>[3x]GHMWPSAKFIDGRVAFSRMPAERELDEVARDFDAVVVLVEDYELPYSLDEWEKRGVEVLHGPIPDFTAPSVEQLLEILRWIEERVREGKKVLIHCMGGLGRSGTVGVAWLMYSRGLSLREALMEVRRKRPGAVETQEQMEVLKELEERI

In this study, we report the crystal structures of three forms of Tk-PTP, which showed that this protein forms a canonical DUSP fold and that it undergoes an atypical temperature-dependent conformational change between two forms. Structural and biochemical analyses revealed that this structural alteration requires the presence of the GG motif in the P-loop, and that Tk-PTP has dual amino acids, Asp63 and Glu132, both functioning as the general acid/base residues. PTP proteins commonly share a highly conserved active site motif called the PTP signature motif, which is also present in Tk-PTP as HC93MGGLGR99. This motif, constituting the phosphate binding loop (or simply called P-loop), contains the catalytic cysteine residue (Cys93) that functions as a nucleophile for dephosphorylation and the conserved arginine residue (Arg99) that anchors the phosphate group of the substrate during the enzyme reaction.

To validate this hypothesis, 0.6 mM purified Tk-PTP protein in the final purification buffer containing 50 mM Tris-HCl (pH 7.5), 200 mM NaCl, and 2 mM dithiothreitol was heated at 60°C for 3 hours to induce its conversion to an enzymatically active form. Simultaneously, sodium vanadate, a widely used PTP inhibitor targeting the catalytic site pocket, was added at a molar ratio of 1:3, to prevent this protein from reverting to the catalytically inactive form during crystallization. Hexagonal prism-shaped crystals were obtained with the heat-treated Tk-PTP protein, and its structure was determined to a resolution of 1.8 Å, referred to as Tk-PTP(form II) in this manuscript. Three molecules of Tk-PTP(form II), which were well matched with each other when superimposed with an RMSD of 0.36−0.38 Å, were contained in the asymmetric unit of the crystal (space group P61). However, the P-loop conformation of Tk-PTP(form II) is quite different from that of Tk-PTP(form I) (an RMSD of 2.39 Å over 8 aligned Cα atoms), with a flip of the Met94−Gly95 peptide bond and a remarkable shift in the main chain backbone atoms of Met94−Leu97. Vanadate is anchored in the active site of Tk-PTP(form II), stabilized by electrostatic interaction with the guanidinium group of Arg109 and by its oxygen atom-mediated hydrogen bonds with the main chain amides of Met94, Gly95, Leu97, Gly98, and Arg99. The Tk-PTP(form II) P-loop is structurally similar to those of catalytically active DUSP proteins such as DUSP23a (an RMSD of 0.29 Å over 8 aligned Cα atoms). Consistently, the main chain amides of the P-loop of Tk-PTP(form II) are directed towards the interior of the active site pocket, similar to those of DUSP3, but remarkably differently to those of Tk-PTP(form I).> CGCGAXUU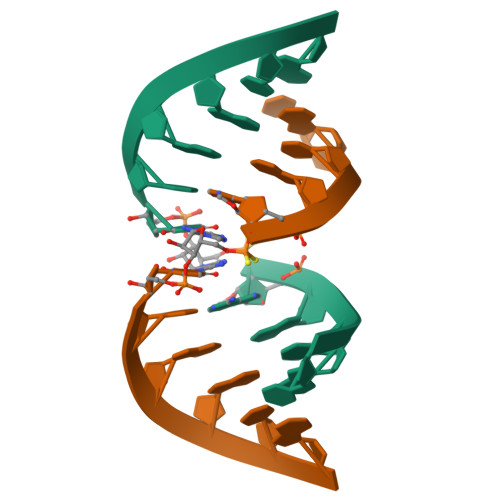AGCG(2~{S})-1-[(2~{S})-2-oxidanylpropoxy]propan-2-ol | C6 H14 O3 | 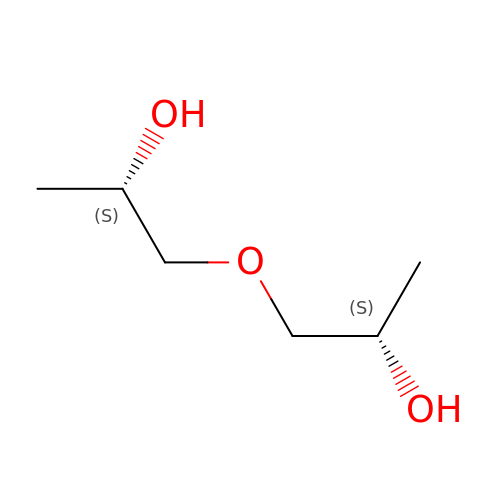AZUXKVXMJOIAOF-WDSKDSINSA-N> MSN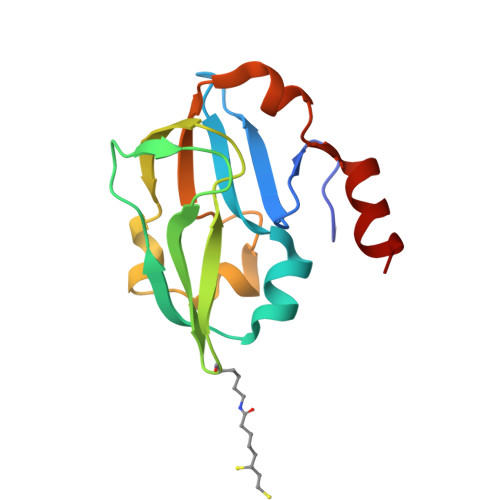VPAELKYSKEHEWLRKEADGTYTVGITEHAQELLGDMVFVDLPEVGATVSAGDDCAVAESVKAASDIYAPVSGEIVAVNDALSDSPELVNSEPYAGGWIFKIKASDESELESLLDATAYEALLEDE>[2x]GPGMKDCSNGCSAECTGEGGSKEVVGTFKAKDLIVTPATILKEKPDPNNLVFGTVFTDHMLTVEWSSEFGWEKPHIKPLQNLSLHPGSSALHYAVELFEGLKAFRGVDNKIRLFQPNLNMDRMYRSAVRATLPVFDKEELLECIQQLVKLDQEWVPYSTSASLYIRPTFIGTEPSLGVKKPTKALLFVLLSPVGPYFSSGTFNPVSLWAN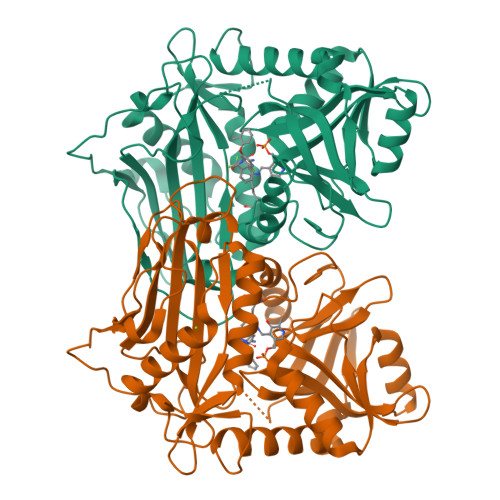PKYVRAWKGGTGDCKMGGNYGSSLFAQCEAVDNGCQQVLWLYGEDHQITEVGTMNLFLYWINEDGEEELATPPLDGIILPGVTRRCILDLAHQWGEFKVSERYLTMDDLTTALEGNRVREMFGSGTACVVCPVSDILYKGETIHIPTMENGPKLASRILSKLTDIQYGREERDWTIVLS>LGSMESTQ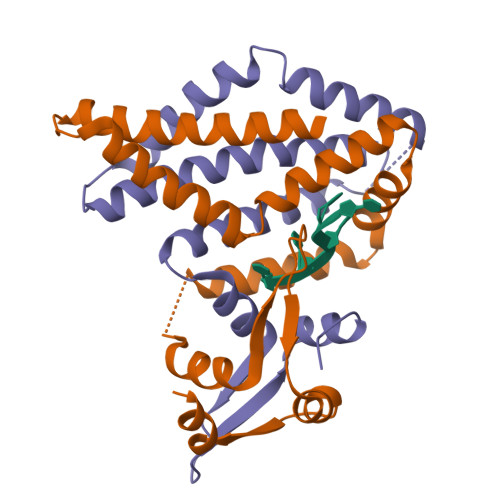QMAVSIINSSFEAAVVAATSALENMGIEYDYQDIYSRVKNKFDFVMDDSGVKNNPIGKAITIDQALNNKFGSAIRNRNWLADTSRPAKLDEDVNKLRMMLSSKGIDQKMRVLNACFSVKRIPGKSSSIIKCTKLMRDKLERGEVEVDDSFVDEKME[8x]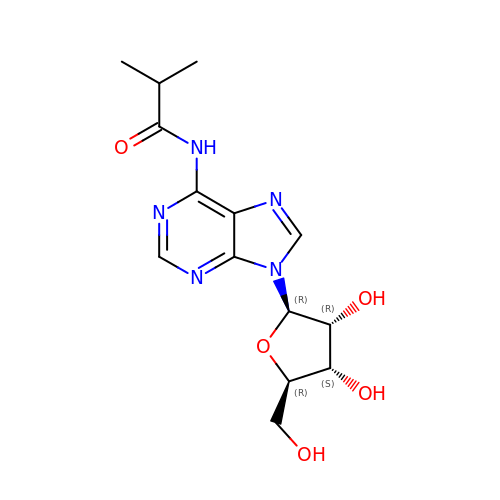N-(2-methylpropanoyl)adenosine | C14 H19 N5 O5 | RSLAEWMJDPSZPS-AKAIJSEGSA-N> EFRPGDKVVLPPYGVGVVAGIAQRSVSGVSRAYYQVDFPGSRSKAYVPVEAPHSVGLRKALAPEEVPVILDLLKNGRMPLPKQWAARHRKTSEILADGNPYRIAQMAGQLRAWEVERGLPDLDRQALRRAIHLLAEEVAQSLEITVQEAKRLF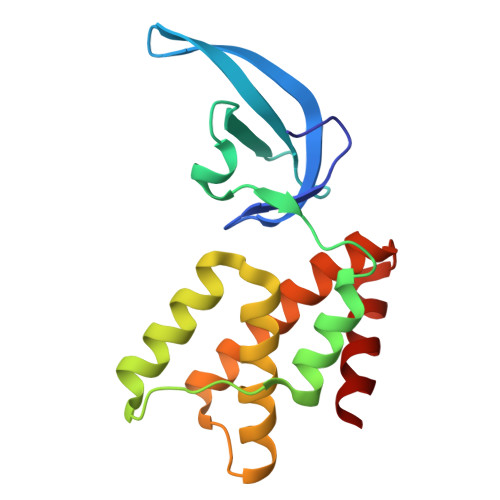EEAWG>[2x]GAC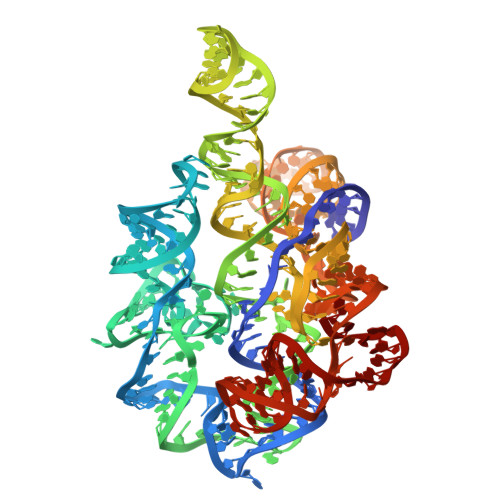CGUCAAAUUGCGGGAAAGGGGUCAACAGCCGUUCAGUACCAAGUCUCAGGGGAAACUUUGAGAUGGCCUUGCAAAGGGUAUGGUAAUAAGCUGACGGACAUGGUCCUAACCACGCAGCCAAGUCCUAAGUCAACAGGAGACUGUUGAUAUGGAUGCAGUUCACAGACUAAAUGUCGGUCGGGGAAGAUGUAUUCUUCUCAUAAGAUAUAGUCGGACCUCUCCCGAAAGGGAGUUGGAGUACUCG> HHSMAAQGPSPIPTNRLKQIAADACNDAIGSAEFYDHAKTEQWNHQIINTILKAVIAESQPSDSTTPPQFKFAVNSTIVQHLVPSSKLNKPAGGADDKPASTATST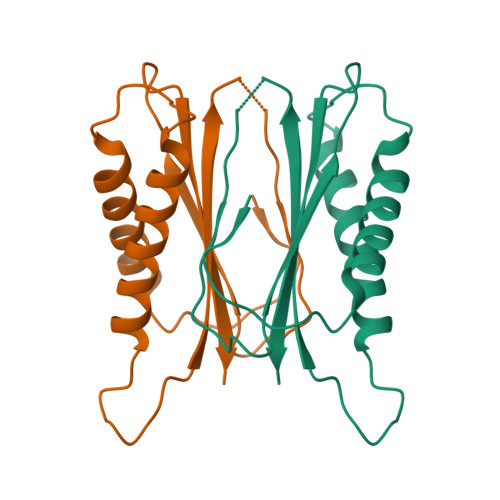DGKPHVGRRGMHSATGAFWNDKTDGMWTYKHEGDESKGMDVVVMLIWIAV>YFPPPAAKEDFLGCLVKEIPPRLLYAKSSPAYPSVLGQTIRNSRWSSPDNVKPLYIITPTQVSHIQSAVVCGRRHSVRIRVRSGGHDYEGLSYRSLQPETFAVVDLNKMRAVWVDGKARTAWVDSGAQLGELYYAIYKASPTLAFPAGVCPTIGVGGNFAGGGFGMLLRKYGIAAENVIDVKLVDANGKLHDKKSMGDDHFWAVRGGGGESFGIVVAWQVKLLPVPPTVTIFKISKTVSEGAVDIINKWQVVAPQLPADLMIRIIAQGPKATFEAMYLGTCKTLTPLMSSKFPELGMNPSHCNEMSWIQSIPFVHLGHRDALEDDLLNRQNSFKPFAEYKSDYVYQPFPKTVWEQILNTWLVKPGAGIMIFDPYGATISATPESATPFPHRKGVLFNIQYVNYWFAPGAAAAPLSWSKDIYNYMEPYVSKNPRQAYANYRDIDLGRNEVVNDVSTYASGKVWGQKYFKGNFERLAITKGKVDPTDYFRNEQSIPP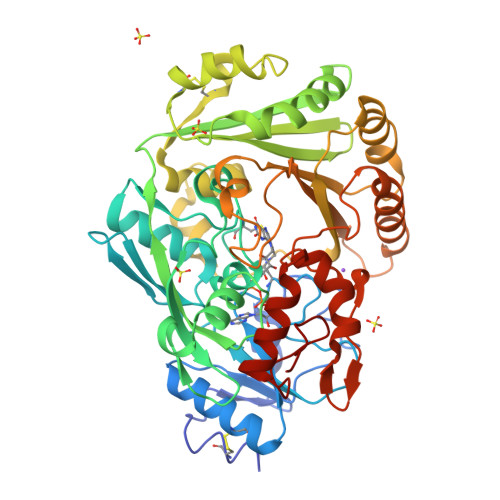LIKKY[2x]> NNDITAENNNIYKAAKDVT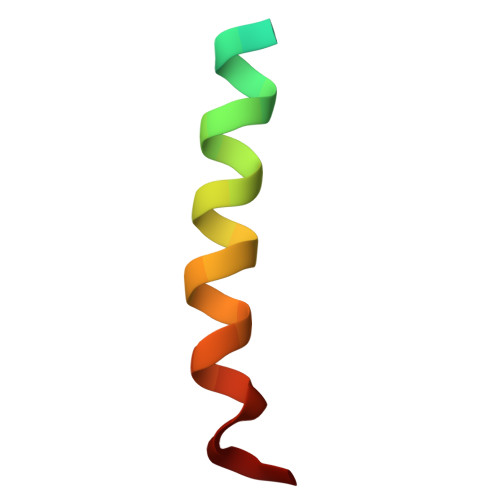TSLSKVLKNIN>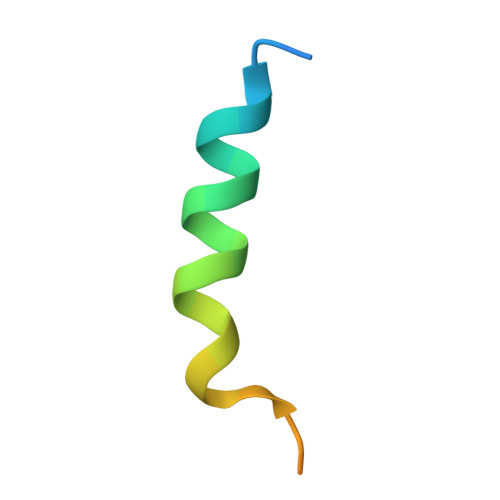 PKFGPYQKALREIRYSLLPFANESGTSAAAEV>MGHHH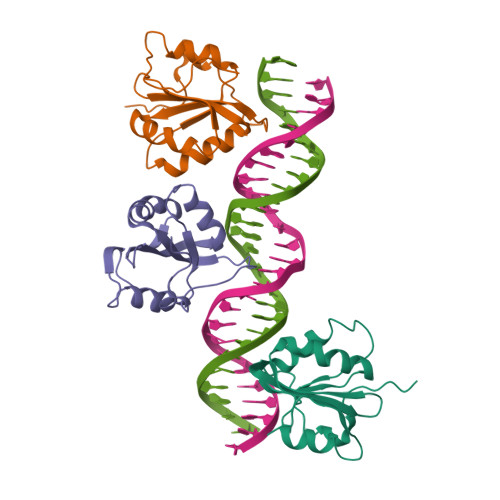HHHGETPVPTDFPIDLSDYLSHAVYSNKTVSCFAIYTTSDKAIELYDKIEKFKVDFKSRHACELGCILLFITLSKHRVSAIKNFCSTFCTISFLICKGVNKMPEMYNNLCKPPYKLLQENKPLLNYEFQE[3x]The best-characterised SAAT, antigen 43 (Ag43), is a protein that contributes to cell aggregation and biofilm formation in commensal Escherichia coli K-12 as well as in major pathotypes including enterohemorrhagic E. coli (EHEC) and uropathogenic E. coli (UPEC). Ag43 possesses a modular domain organisation that is common throughout the ATs, which encompasses an N-terminal signal sequence that directs the secretion of the protein across the inner membrane, a passenger (α) domain that is responsible for the function of the protein, and a C-terminal translocator (β) domain that facilitates the translocation of the functional α-domain to the cell surface. After translocation, the Ag43 α-domain (α43) is cleaved but remains attached to the cell via non-covalent interactions. Similar to α43a 13, the α-domain of all three Ag43 variants folds into an L-shaped right-handed three-stranded β-helix, with each turn of the β-spine comprising three β-strands linked by loop regions.

α43_EDL933 crystals belonged to the space group P212121, diffracting to 2.98 Å and contained four molecules per asymmetric unit. The α43_UTI89 and α43_EDL933 structures in this work correspond to the uncleaved α-domains. Present within the structures of α43_UTI89 and α43_EDL933, their AC regions consist of three β-strand rungs capped by a β-hairpin motif. The first superposition predicted an α43_EDL933 functional dimer stabilised by two interfaces, each consisting of 12 hydrogen bonds. Conversely, when the α43_UTI89 functional dimer was used as the scaffold, α43_EDL933 molecules were predicted to self-associate via one interface also encompassing 24 hydrogen bonds. We generated a second mutant where we mutated T199 and T256 to glycine at the base of α43_EDL-933 (Ag43EDL933-mt-double), mapping far from the predicted single interface, and responsible for 10 out of the total predicted 24 hydrogen bonds stabilising the putative Ag43EDL933 double interface dimer. Examination of MS528 strains expressing these mutants in cell-aggregation assays showed that while modification of the predicted Ag43EDL933 single interface did not alter its aggregative function, mutation of two residues in the double interface completely abolished Ag43EDL933 mediated cell aggregation. Hence, we confirmed that α43_EDL933 interacts via an extensive double interface. Although both dimers are possible, the double interface dimer results in a 550 Å2 buried surface area, compared to 260 Å2 for the single interface dimer, suggesting that interactions such as van der Waals contacts are also important for dictating the preference for the double interface dimer.

>SNAADKVVQAGETVNDGTLTNHDNQIVFGTANGMTISTGLELGPDSEENTGGQWIQNGGIAGNTTVTTNGRQVVLEGGTASDTVIRDGGGQSLNGLAVNTTLNNRGEQWVHEGGVATGTIINRDGYQSVKSGGLATGTIINTGAEGGPDSDNSYTGQKVQGTAESTTINKNGRQIILFSGLARDTLIYAGGDQSVHGRALNTTLNGGYQYVHRDGLALNTVINEGGWQVVKAGGAAGNTTINQNGELRVHAGGEATAVTQNTGGALVTSTAATVIGTNRLGNFTVENGKADGVVLESGGRLDVLESHSAQNTLVDDGGTLAVSAGGKATSVTITSGGALIADSGATVEGTNASGKFSIDGTSGQASGLLLENGGSFTVNAGGQAGNTTVGHRGTLTLAAGGSLSGRTQLSKGASMVLNGDVVSTGDIVNAGEIRFDNQTTPNAALSRAVAKSNSPVTFHKLTTTNLTGQGGTINMRVRLDGSNASDQLVINGGQATGKTWLAFTNVGNSNLGVATTGQGIRVVDAQNGATTEEGAFALSRPLQAGAFNYTLNRDSDEDWYLRSEN[4x]Dimethylallyl 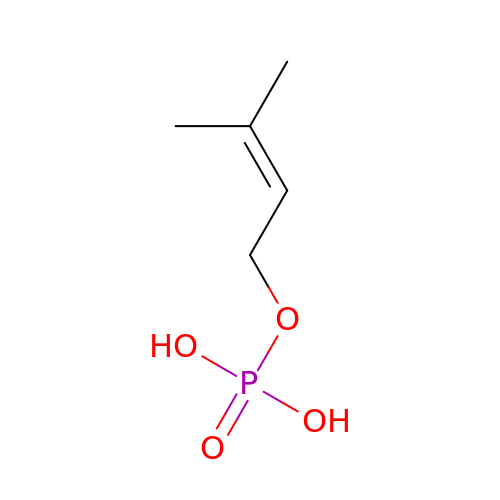monophosphate | C5 H11 O4 P | MQCJHQBRIPSIKA-UHFFFAOYSA-N>[8x]MAATRTRGYV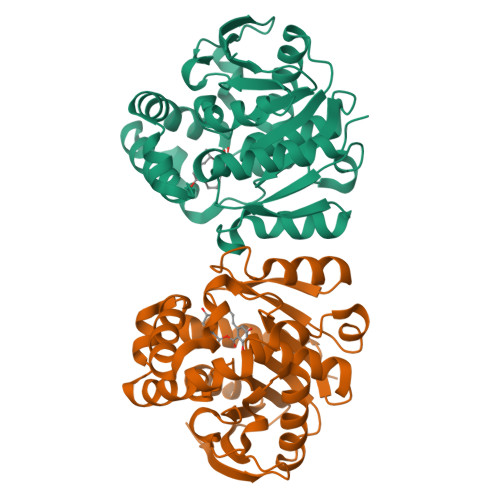TTKDGIKWYYEQEGSGPDVVLIPDGLGECQMFDKPMSLIASNGFRVTTFDMPGMSRSSDAPPETYQDITGRKLAGYIITLLDTLDIKIASVWGCASGASTVLALCSDYPERVRNGMPHEVPTENPDILLHIHEVDPATISQEMAANSRAYSGNVEAWDALGPEVHARLHDNYPRWAYGYPRTIPPSAPVKTEDLHKVPIDWTVGASTPTKLFFENIVIAAREGINIGTLPGNHFPYVSHPEEFAKYVVETSRKYLK>[2x]GKKEFLKHEYSPGHWSIDYTRAGTSIAVITVRNKYHYSVILNPTDCRGYRIIIRYLNEGDST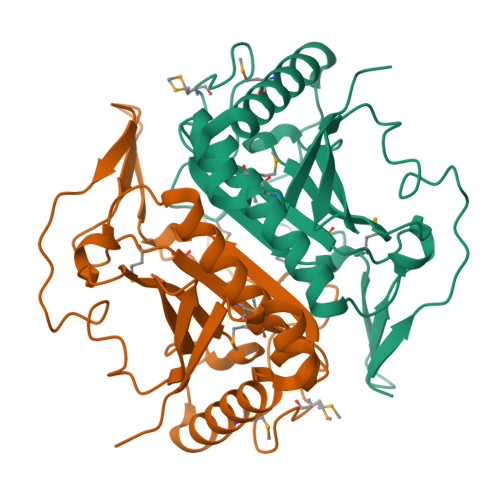LSSAFNRPYTVSEQRGLNDVASLMTQVYEKLGLIVQFSQLGNNSQSFDKGTGVTLIGSEEEPSMLHLHMWGRGDPDMEYIAGVPLRGPEPGLMFDLIAKNKTHPINQHAIKWNEEELKACLAMFKLKLAEYVNSPEFTEEFGDTLKVTIHDKK>GPGNNELSPVALRQMSCAAGTTQTACTDDNALAYYNTTKGGRFVLALLSDLQDLKWARFPKSDGTGTIYTELEPPCRFVTDTPKGP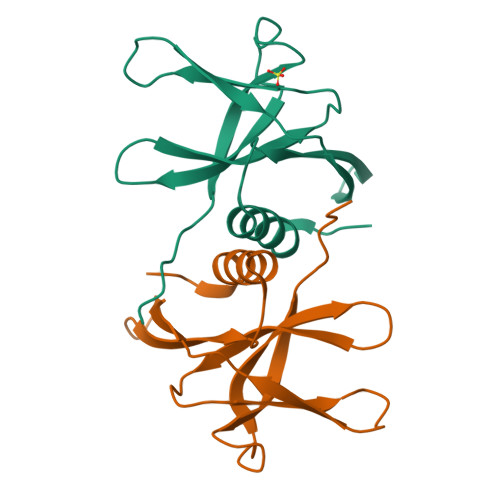KVKYLYFIKGLNNLNRGMVLGSLAATVRLQ[2x]> GPLGSMKLLVVDDSSTMRRIIKNTLS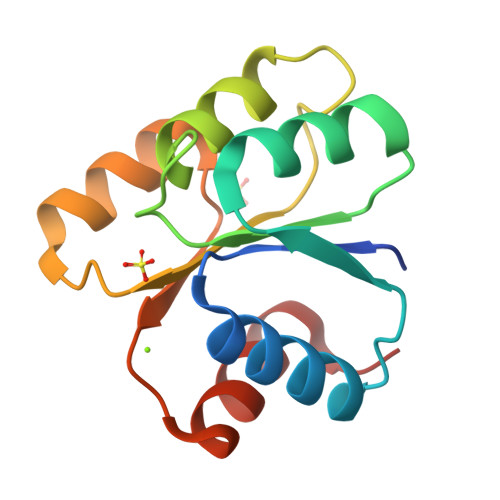RLGYEDVLEAEHGVEAWEKLDANADTKVLITAWNMPEMNGLDLVKKVRSDSRFKEIPIIMITTEGGKAEVITALKAGVNNYIVKPFTPQVLKEKLEVVLGTND> SNASQEEKFAETYNETTAFNNKVDGSAVQLVSDKADKAKTVDIYEDFSCHYCSQLAKETDADMKKLIEDGKVKVNIRTMNFLDKGEIGHSNKAGTAAYTIAKDDSAQVYWNFRTMLMTEQQNIWGKKELKDLADMAKILGAKDETVKKIADGTYSDEFKKIADDNAKKLEKDGDGQVSSPRVFID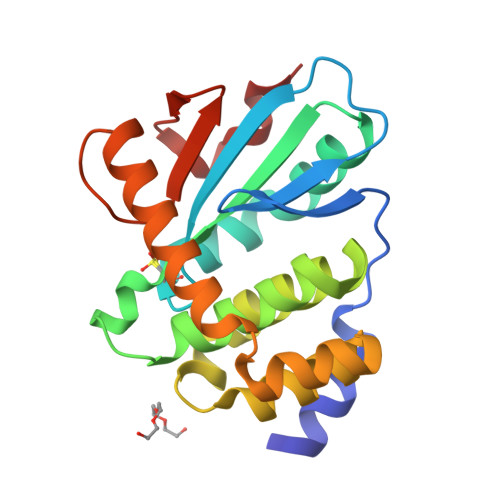GKEIKENATWPSQIK3-Chloro-N-[2-(2,4-dioxo-1,3-thiazolidin-3-yl)ethyl]benzamide 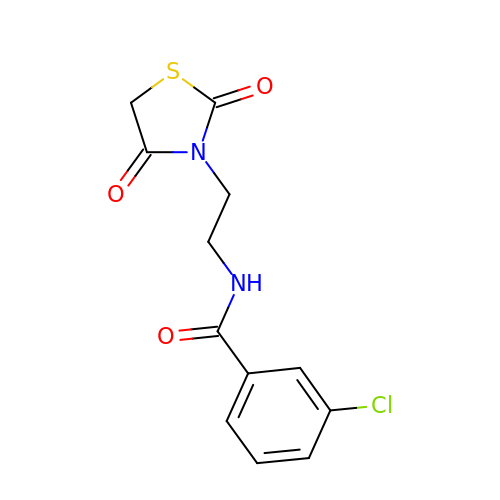| C12 H11 Cl N2 O3 S | CWILDSFKHIQHCJ-UHFFFAOYSA-N2,6-DIHYDROANTHRA/1,9-CD/PYRAZOL-6-ONE 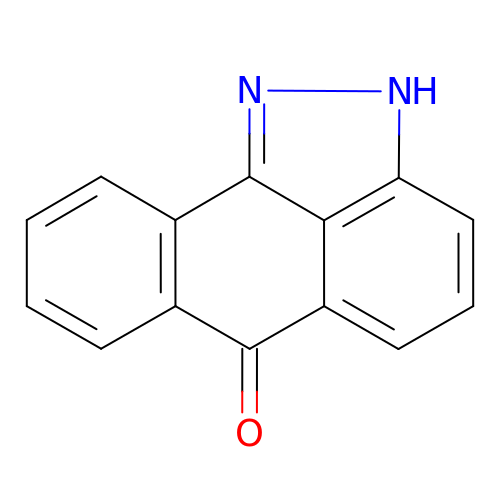| C14 H8 N2 O | ACPOUJIDANTYHO-UHFFFAOYSA-N>[6x]GAMAVTTVGFDVAARLGTLLTAMVTPFSGDGSLDTATAARLANHLVDQGCDGLVVSGTTGESPTTTDGEKIELLRAVLEAVGDRARVIAGAGTYDTAHSIRLAKACAAEGAHGLLVVTPYYSKPPQRGLQAHFTAVADATELPMLLYDIPGRSAVPIEPDTIRALASHPNIVGVKDAKADLHSGAQIMADTG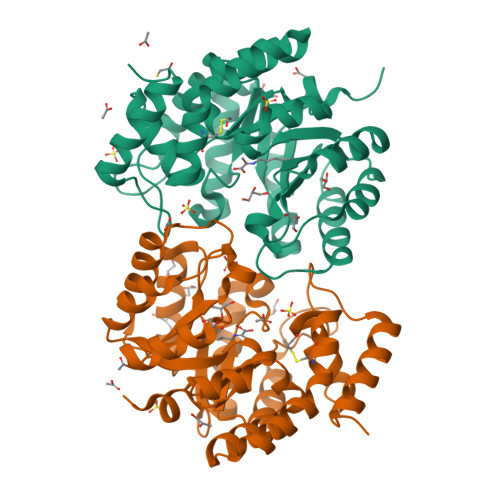LAYYSGDDALNLPWLRMGATGFISVIAHLAAGQLRELLSAFGSGDIATARKINIAVAPLCNAMSRLGGVTLSKAGLRLQGIDVGDPRLPQVAATPEQIDALAADMRAASVLR> GPLGSNEEANRFANQAKLRVQEAVFYIWSDKTLKYSQM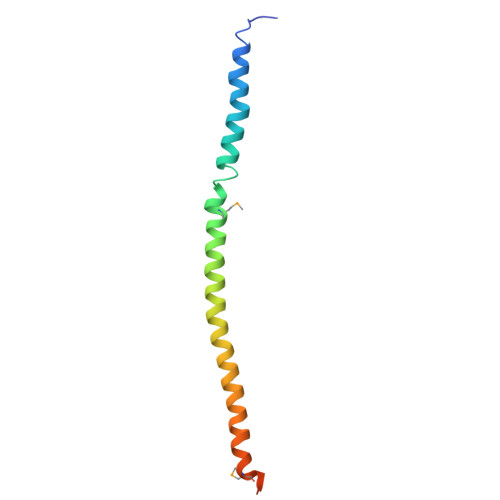ANDEAESFRNTWLLFRSFQQWITLTQTFKEQSRLADQAFLNKMFRKILKAQEHWKH>[8x]MDIITKMQVDVPRETVFEAFVDPEKIGGFWFSSSSERWEQGKTITLRYEEYDAELNINIERVEDNQLIAFTWGAHPITIQFEESEAGTVVTTTEKDFDTQDVKQLLGQKEGWVYM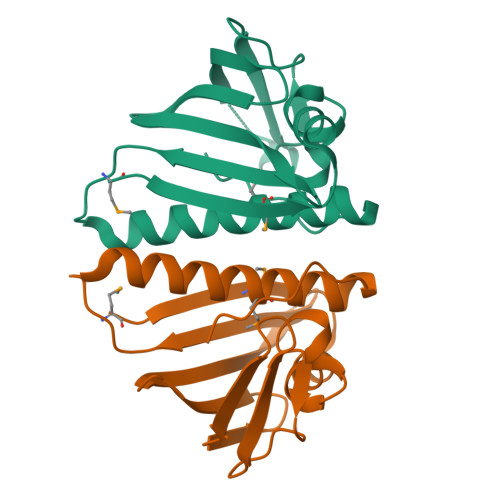LSCLKVYLEHGVTIRAAILL>HHMGNLNRCIADIVSLFITVMDKLRLEIRAMDEIQPDLRELMETMNRMSHLPPDFEGREKVSQWLQKL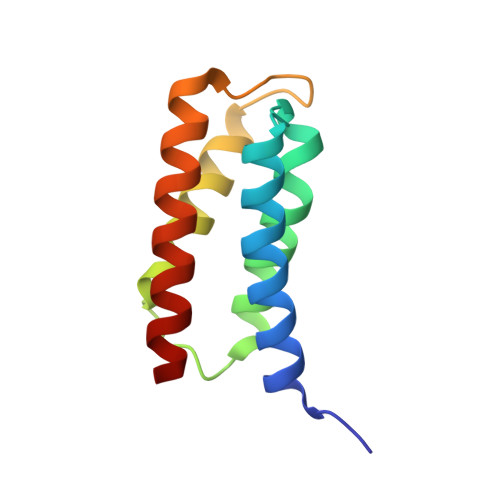SSMSASDELDDSQVRQMLFDLESAYNAFNRFLHS[2x]> SMGESRVILAFGDSLFAGYGLDKGESYPAKLETALRSHGINARIINAGVSGDTTAAGLQRIKFVLDSQPDKPELAIVELGGNDLLRGLSPAEARQNLSGILEELQRRKIPILLMGMRAPPNLGAKYQ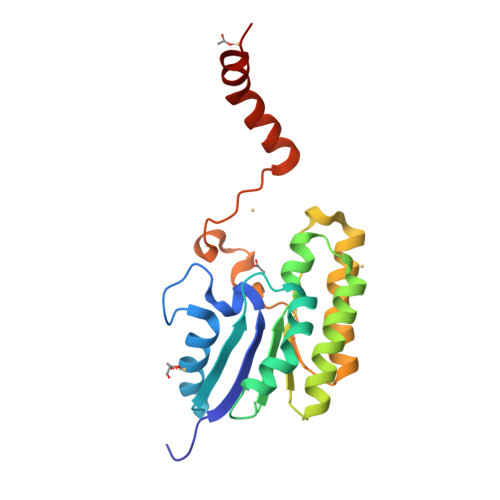REFDGIYPYLAEKYDAKLVPFFLEAVADRPDLIQKAHVHPTARGVEELVSATSNAVAKALPAKK> GPLGSEKIEKDNAFAFDLLQTTRKHVTEANVFISPLSVSMALNMTLNGAAGVTADEMKTALRETGYTMEDINEYSHSLREALLKVDPSTTIGMANSIWYKQGELVKEPFILANRTHYDAEVKAVDFSSPATLPAINGWCAQKTNDKITKILDYIPGNAFMYLINAVYFKGIWVTQFKKSDTKRAPFRKA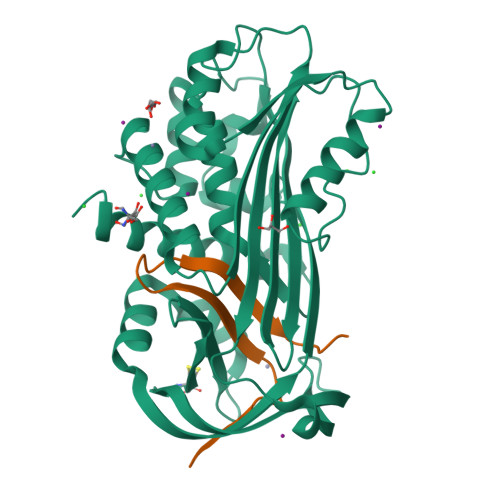DGTTQEVNMMAQKSTFGYTTDECCQYLEMDYGNKAFSMIVMLPNEGQTTRDVIEQLDNKHWSMIIKGIRPTQVSLRMPRFKTECKYGLEKKILPEMGMNVPFTETADFPGITDAAIFISRVIHKTFVQVDEEGTEAAAVTAVEMK;> ATSSPSTTPINFHINKPFVFAIREKSTGVILFIGEIGEVKE>GSHMTKITLSDLPLREELRGEHAYGAPQLNVDIRLNTNENPYPPSEALVADLVATVDKIATELNRYPERDAVELRDELAAYITKQTGVAVTRDNLWAANGSNEILQQLLQAFGGPGRTALGFQPSYSMHPILAKGTHTEFIAVSRGADFRIDMDVALEEIRAKQPDIVFVTTPNNPTGDVTSLDDVERIINVAPGIVIVDEAYAEFSPSPSATTLLEKYPTKLVVSRTMSKAFDFAGGRLGYFVANPAFIDAVMLVRLPYHLSALSQAAAIVALRHSADTLGTVEKLSVERVRV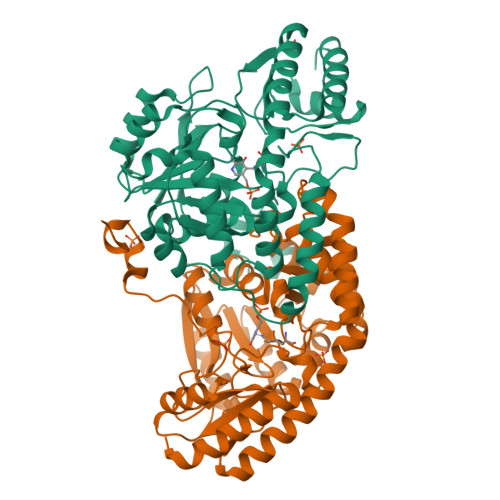AARLEELGYAVVPSESNFVFFGDFSDQHAAWQAFLDRGVLIRDVGIAGHLRTTIGVPEENDAFLDAAAEIIKLNL[3x]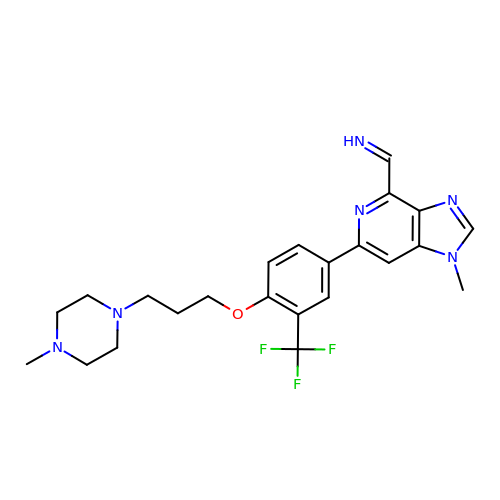(E)-1-(1-methyl-6-{4-[3-(4-methylpiperazin-1-yl)propoxy]-3-(trifluoromethyl)phenyl}-1H-imidazo[4,5-c]pyridin-4-yl)methanimine | C23 H27 F3 N6 O | MZJARPQAOGJEES-MZJWZYIUSA-N The nucleocapsid (N) protein plays critical roles in coronavirus genome transcription and packaging, representing a key target for the development of novel antivirals, and for which structural information on ligand binding is scarce. The NTD is implicated in the binding and melting of regulatory elements required for transcription initiation, whereas the CTD drives protein dimerization and is thought to contribute to the binding of the RNA packaging signal (PS) sequence during virus particle assembly.

Six molecules organized as three dimers were found in the asymmetric unit of the CTD. Each protomer in the structures is comprised of five α-helices, two 310 (η) helices and two antiparallel β-strands. The CTD dimer is stabilized by extensive hydrogen bonds connecting the β2 strands (Leu331–Ile337) and the interaction of residues from the loop between α-helices 1–2 (Arg277, Gly278, Glu280, Gln283 and Asn285). β-strand 1 and α-helix 4 (Gly316, Arg319 and Ile320) also play an essential role in stabilizing the dimer. The CTD structure in its apo form shows an electrostatic potential distribution that is conserved amongst all N proteins from the Coronaviridae family, with a major positively charged groove located on one side of the dimer surface. This region—which is flanked by Lys256 and Lys257 from both protomers in a CTD dimer and further composed by Lys259, Lys261 and Arg262—is thought to contribute to RNA binding. We observed that this positively charged groove extends towards the CA-binding pocket through Arg259, Arg276, Arg277 and Arg293. When the apo and complexed structures were superposed, we observed no significant changes in the overall structures, as judged by the Cα RMSD (0.19 Å deviation).

>[6x]AAEASKKPRQKRTATKAYNVTQAFGRRGPEQTQGNFGDQELIRQGTDYKHWPQIAQFAPSASAFFGMSRIGMEVTPSGTWLTYTGAIKLDDKDPNFKDQVILLNKHIDAYKTFP>MGVDPLNDPNSPLAKRSIYFDFDSYSVKDEYQPLMQQHAQYLKSHPQRHVLIQGNTDERGTSEYNLALGQKRAEAVRRAMALLGVNDSQMEAVSLGKEKPQATGHDEASWAQNRRADLVYQQLEHHH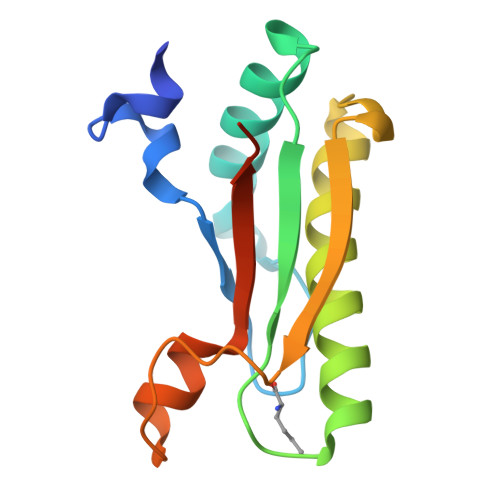HHH[2x]>MTSAASYDFKFMSYMVNKAKSVNKALEEAVPLREPELKIREAMRYTLLSDGKRVRPMLCLAACELVGGQESTAMSAACAIEMLHASSLILDDLPCMDNDSLRRGKPTNHIVFGESIAILASQALIALAVQKTTSSTFADVPPERILKTVQEMVKAVEGLVAGQQADLAGEGMRFDSDTGLEHLEFIHIHKTAALLEAAAVMGAIMGGGSDEEIERLRSYARCIGLMFQVVDDVLDVTKSSEELGKTAGKDLIAGKLTYPRLMGVEKS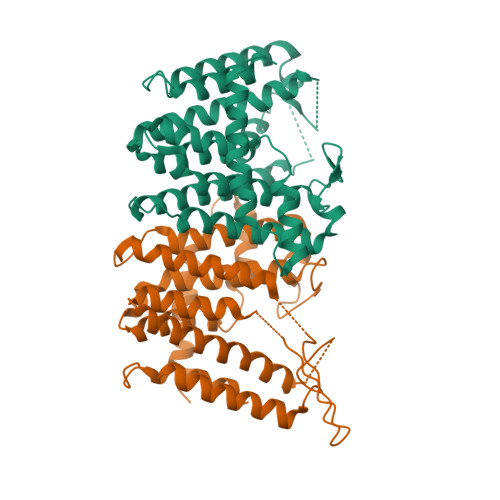KEYAERLNIEAREHLLGFDIDKVAPLVSLADYIVNRQNLEHHHHHH[2x]> GDSSMSYKIPVHADFLIAYSTVPGFYSWRNTTRGSWFMQSLCAELAANGKRLDILTLLT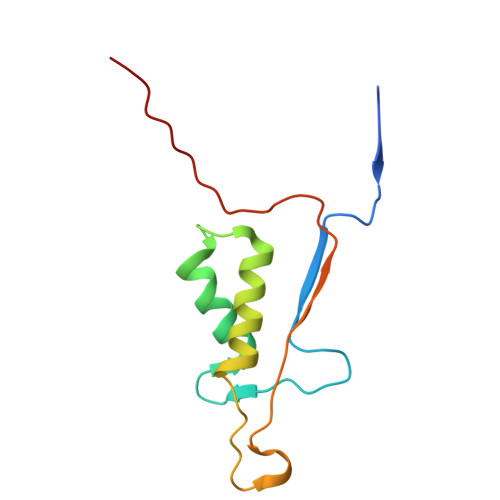FVCQRVAVDFESCTPDTPEMHQQKQIPCITTMLTRILRFSDKQLAPAGRV[[(2~{R},3~{S},4~{R},5~{R})-5-(6-aminopurin-9-yl)-3,4-bis(oxidanyl)oxolan-2-yl]methoxy-oxidanyl-phosphoryl] 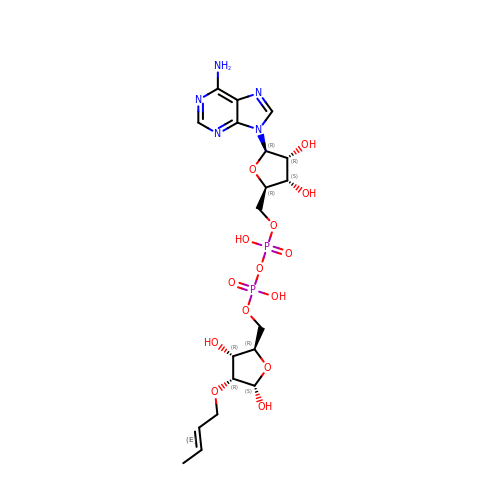[(2~{R},3~{R},4~{R},5~{S})-4-[(~{E})-but-2-enoxy]-3,5-bis(oxidanyl)oxolan-2-yl]methyl hydrogen phosphate | C19 H29 N5 O14 P2 | JOKNWQJJLFYBKK-YVAUJSGTSA-N>GSHMFTSLEGRSAIVTGGSKGIGRGIAETFANAGVDVVITGRNQDDLDRTVADLS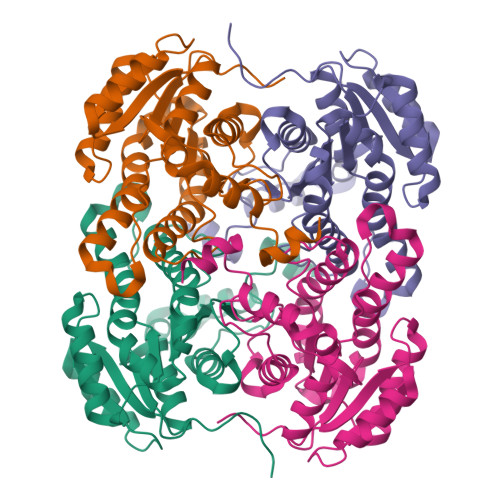GTRGKVTAVRADVTDPEDARRTVAETVSRHGGLDIVCANAGIFPSGRLEDLTPDDIEQVLGVNFKGTVYIVQAALQALTASGHGRVVVTSSITGPITGYPGWSHYGASKAAQLGFLRTAAMELAPKKITINAVLPGNIMTEGLDEMGQDYLDQMASAIPAGRLGSVADIGNAALFFATDEAAYVTGQTLVVDGGQVLPESHLAIAEL[2x]>[18x]MTAVSEFRPGLEGVPATLSSISFVD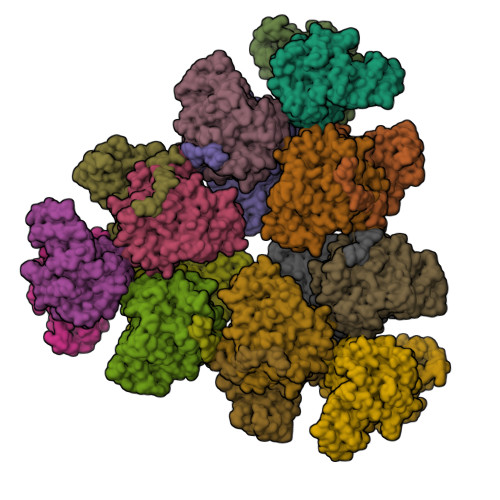GQRGVLEYRGISIEQLAQQSSFLETAYLLIWGHLPTQQELTEFEHEIRYHRRIKFRIRDMMKCFPDSGHPMDALQASAAALGLFYSRRALDDPEYIRAAVVRLLAKIPTMVAAFQLIRKGNDPIQPRDELDYAANFLYMLTEREPDPVAARIFDICLTLHAEHTINASTFSAMVTASTLTDPYAVVASAVGTLAGPLHGGANEEVLDMLEAIGSVENVEPYLDHCIATKTRIMGFGHRVYKVKDPRAVILQNLAEQLFDIFGHDPYYEIAVAVEKAAAERLSHKGIYPNVDFYSGLVYRKLGIPSDLFTPVFAIARVAGWLAHWKEQLNENRIFRPTQIYTGSHNLDYTPIADRDLAIESDLEHHHHHH>[4x]MTSASNPPAFRLETSDGDEEGSAEVNKGKNEPPPMESPFQGEDRNFSPQIKVNLNYRKGLGPSQQDPNRFDRDRLFSVVSR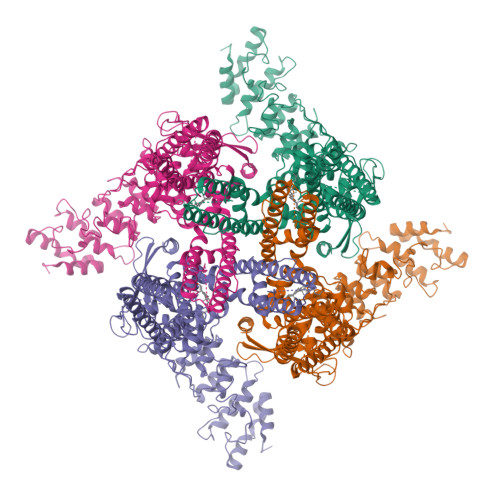GVPEELTGLLEYLRRTSKYLTDSAYTEGSTGKTCLMKAVLNLQDGVNACILPLLQIDRDSGNPQPLVNAQCTDEFYRGHSALHIAIEKRSLWCVKLLVENGANVHIRACGRFFQKHQGTCFYFGELPLSLAACTKQWDVVTYLLENPHQPASLEATDSLGNTVLHALVMIADNSPENSALVIHMYDSLLQMGARLCPTVQLEDICNHQGLTPLKLAAKEGKIEIFRHILQREFSGLYQPLSRKFTEWCYGPVRVSLYDLSSVDSWEKNSVLEIIAFHCKSPHRHRMVVLEPLNKLLQEKWDRLIPRFFFNFACYLVYMIIFTIVAYHQPSLEQPAIPSSKATFGDSMLLLGHILILLGGIYLLLGQLWYFWRRRLFIWISFMDSYFEILFLVQALLTVLSQVLRFVETEWYLPLLVSSLVLGWLNLLYYTRGFQHTGIYSVMIQKVILRDLLRFLLVYLVFLFGFAVALVSLSREARSPKAPEDSNTTVTEKPTLGQEEEPVPYGGILDASLELFKFTIGMGELAFQEQLRFRGVVLLLLLAYVLLTYVLLLNMLIALMSETVNSVATDSWSIWKLQKAISVLEMENGYWWCRRKRHRAGRLLKVGTKGDGIPDERWCFRVEEVNWAAWEKTLPTLSEDPSGAGITGYKKNPTSKPGKNSASEEDHLPLQVLQSH>[5x]MDLAPQMLRELQETNAALQDV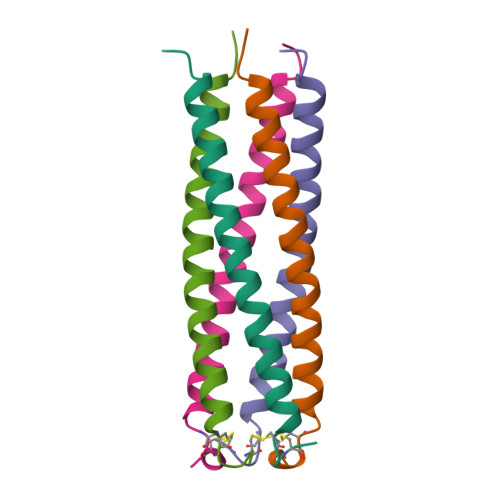RELLRQQVKEITFLKNTVMECDACG>[2x]MPKKTIFFGAGWFTDRQNKAYKEAMEALKENPTIDLENSYVPLDNQYKGIRVDEHPEYLHDKVWATATYNNNLNGIKTNDIMLGVYIPDEEDVGLGMELGYALSQGKYVLLVIPDEDYGKPINLMSWGVSDNVIKMSQLKDFNFNKPRFDFYEGAVY

A major challenge in the further development of nucleoside analogues for therapeutic applications is access to scalable and environmentally sustainable synthetic strategies. This study uses the type II nucleoside 2′-deoxyribosyltransferase from Lactobacillus leichmannii (LlNDT-2) to prepare a suite of ribonucleoside analogues using naturally-occurring uridine and cytidine sugar donors. An enzymatic alternative to the use of NPs to prepare ribonucleoside analogues is to use nucleoside 2′-deoxyribosyltransferases (NDTs). These enzymes catalyse the formation of nucleoside analogues via an overall nucleobase exchange much akin to NPs. However, NDTs are mechanistically distinct, forming a covalent adduct within the active site, thus controlling stereoselective nucleophilic attack of the incoming nucleobase on the β face.

To gain further insight into how the presence of a 2′-OH substituent on the ribonucleoside donor influences substrate recognition and subsequent catalytic steps, structural studies were conducted on the wildtype LlNDT-2 and a double mutant Y7F/D72N. These two mutations were chosen based on the enhanced acceptance of a ribonucleoside donor in an enzymatic transglycosylation reaction by an analogous double mutant of a type I NDT derived from Trypanosoma brucei (TbNDT). To explore the structural implications of the differences between the two enzymes, WT-LlNDT-2 and the Y7F/D72N mutant were both crystallised using conditions determined for the WT-LlNDT-2 enzyme previously. Complexes were obtained by soaking cytidine 8 into the crystals. All structures contained two molecules in the asymmetric unit, constituting one third of the hexamer routinely observed in solution. In the case of WT-LlNDT-2, electron density in the omit maps obtained could be clearly modelled as the ribosylated intermediate, and the cleaved cytosine nucleobase, whereas in the Y7F/D72N structure cytidine 8 was intact, presumably reflective of its poorer kcat as observed for CtNDT. However, the side chain of N72, which, like that of D72 in the WT-LlNDT-2, forms an interaction with the O2 of cytosine, has different rotamer conformations in each monomer in the asymmetric unit, one of which permits two interactions with cytidine. In addition, in the Y7F/D72N structure, the interactions between the nucleobase of 8 and the side chain of Q46 are slightly different, with the interaction between the nitrogen of the amide and the O2 of 8 observed in the WT complex disrupted by a movement of the Q46 side chain. The interaction between E98 and the 2′-OH alone would militate against the activity of E98 as a nucleophile for attack at C1′ of the substrate; additionally, the even lower activity of the Y7F/D72N mutant versus the WT-LlNDT-2 for ribonucleosides would be compromised by the removal of the interaction between the phenol of Y7 and E98, which may suppress the ionisation of E98 for nucleophilic attack at C1.>[2x]STLQFKVGPPFELVRDYCPVVESH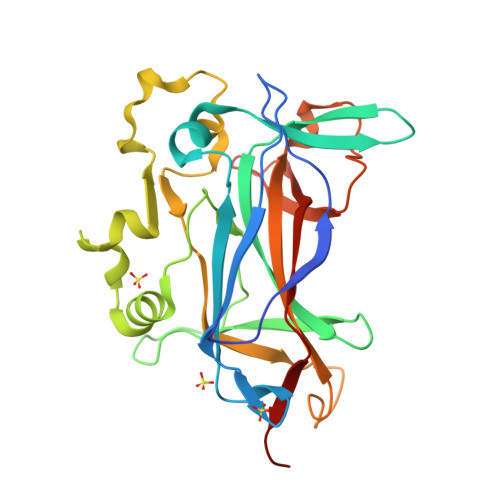TGRTLDLRIIPRIDRGFDHIDEEWVGYKRNYFTLVSTFETANCDLDTFLKSSFDLLVEDSSVESRLRVQYFAIKIKAKNDDDDTEINLVQHTAKRDKGPQFCPSVCPLVPSPLPKHQIIREASNVRNITKTKKYDSTFYLHRNHVNYEEYGVDSLLFSYPEDSIQKVARYERVQFASSISVKKPFQQNKHFSLHVILGAVVDPDTFHGENPGIPYDELALKNGSKGMFVYLQEMKTPPLIIRGRSPSN>MSDIKAVAQRALSLMDLTSLTNTETDQEIIDLCRQAKSPAGET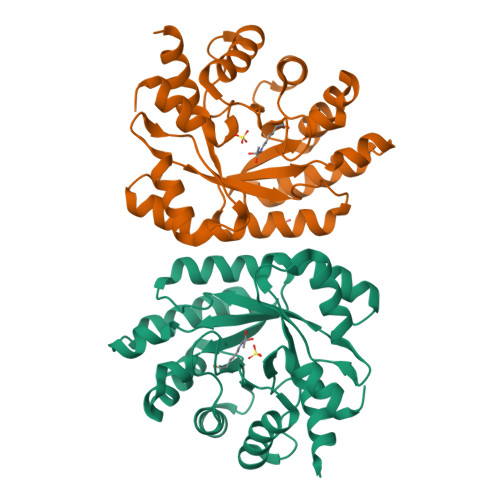AAICIFPRFIPVAKKALKAQQTPHIKIATVTNFPQGNDDLDIALAETRAAVAYGADEVDLVFPYRALIQGNETIGFDMVKVCKQACSGNAKLKVIIETGELKSEELIRKASEIAINAGADFIKTSTGKVAINATPEAAKVMLTVIKNKNTAVGFKPAGGVRNADDAAIYLDLADNILGNEWADANHFRFGASSLLISLLDTLGHKSNTKSSSNYHHHHHH[2x]>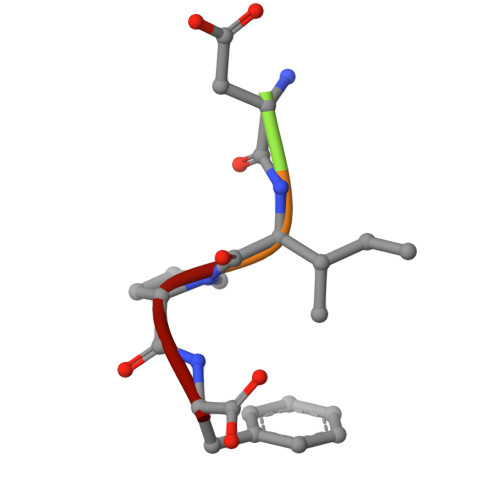 WDIPF(2S)-2-[(1R)-1-{[(2R)-2-amino-2-phenylacetyl]amino}-2-oxoethyl]-5-methyl-3,6-dihydro-2H-1,3-thiazine-4-carboxylic acid | C16 H19 N3 O4 S | 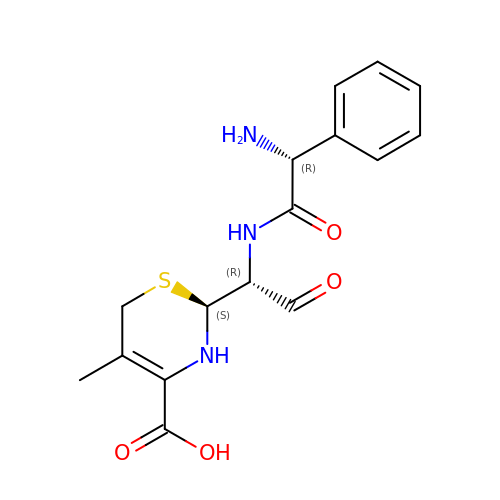YUNPQAOWKVWRNR-JMSVASOKSA-N> DRHHHHHHKLYGRLTRDKKFQRYLARVTDIEATDTNNPNVNYGIVVDCGSSGSRVFVYCWPRHNGNPHDLLDIRQMRDKNRKPVVMKIKPGISEFATSPEKVSDYISPLLNFAAEHVPRAKHKETPLYILCTAGMRILPESQQKAILEDLLTDIPVHFDFLFSDSHAEVISGKQEGVYAWIGINFVLGR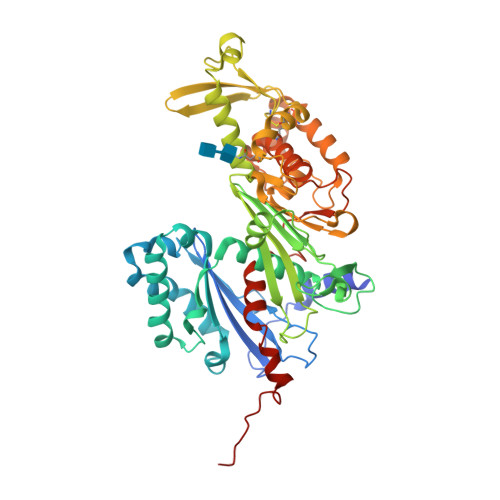FEHIEDDDEAVVEVNIPGSESSEAIVRKRTAGILDMGGVSTQIAYEVPKTVSFASSQQEEVAKNLLAEFNLGCDVHQTEHVYRVYVATFLGFGGNAARQRYEDRIFANTIQKNRLLGKQTGLTPDMPYLDPCLPLDIKDEIQQNGQTIYLRGTGDFDLCRETIQPFMNKTNETQTSLNGVYQPPIHFQNSEFYGFSEFYYCTEDVLRMGGDYNAAKFTKAAKDYCATKWSILRERFDRGLYASHADLHRLKYQCFKSAWMFEVFHRGFSFPVNYKSLKTALQVYDKEVQWTLGAILYRTRFLPLRDIQQEAFRASHTHWRGVS>GPMTADAPAGTLAQPGGISDPNLIKLVNKLQDVFTTVGVNNPIDLPQIVVVGSQSSGKSSVLENIVGRDFLPRGQGIVTRRPLVLQLINRQSSGNANGFDERLADSTDKAANLDEWGEFLHLPGQKFYDFNKIRDEINRETEAKVGRNAGISPAPINLRIYSPHVLNLTLVDLPGLTRVPVGDQPRDIERQIRDMILKYIQKPNAIILAVTAANVDLANSDGLKLAREVDPEGQRTIGVLTKVDLMDEGTDVVDILAGRIIPLRLGYV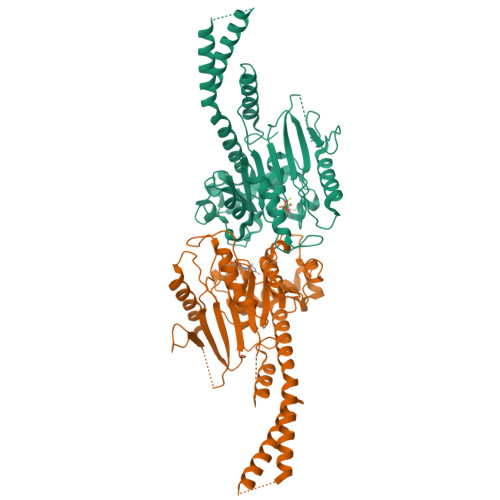PVVNRGQRDIDNKKPITAALEAEKAFFENHKAYRNKSAYCGTPYLARKLNLILMMHIKQTLPDIKQRISSSLQKYQQELEALGPSLLGAGAGAESDYTVRRRKECQQMVESLQRAAEIVSQVQ[4x]> GPLGSEDDLYRQSLEIISRYLREQATGSKD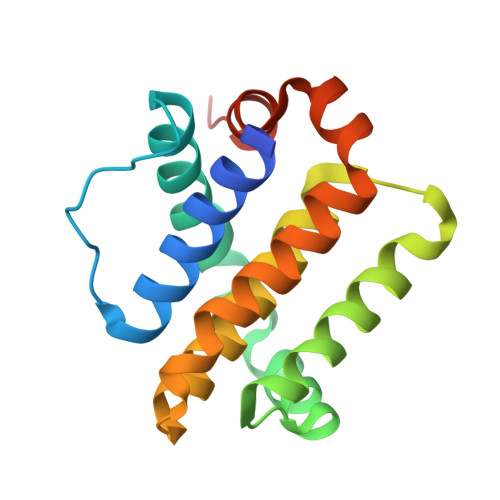SKPLGEAGAAGRRALETLRRVGDGVQRNHETAFQGMLRKLDIKNEDDVKSLSRVMIHVFSDGVTNWGRIVTLISFGAFVAKHLKTINQESCIEPLAESITDVLVRTKRDWLVKQRGWDGFVEFFHVEDLEGG> GGVRGSLGSPGNRENKEKKVFISLVGSRGLGCSISSGPIQKPGIFISHVKPGSLSAEVGLEIGDQIVEVNGVDFSNLDHKEAVNVLKSSRSLTISIVAAAGRE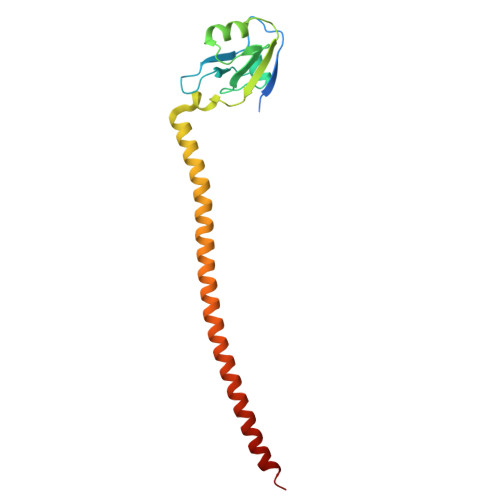LFMTDRERLAEARQRELQRQELLMQKRLAMESNKILQEQQEMERQRRKEIAQKAAEENERYRKEMEQIVEEEEKF>[2x]MQTEYRTASDGSLNWGFRQSFRNYIQTGVAKGSITLGDGASDNGGNFAFTPRTNGTTVTSDSQGTVEF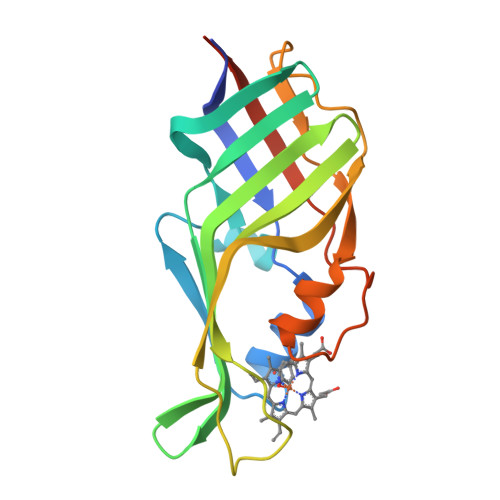NGSVHFLGHQAEDKWILDTTMSDIKMVFNGSSAQLVVDLVAREFKGTTYDDIGEYIISDDIVLADVSLNSAADFSQDSIDLSGTTDLTAAGAQAFGGFYETGEALDPTGGSLTISSTLEHHHHHH>[2x]MGSSHHHHHSSGLVPRGSHMQMIAEIYYERGTIVVKGDAHVPHAKFDSRSGTYRALAFRYRDIIEYFESNGIEFVDNAADPIPTPYFDAEISLRDYQEKALERWLVDKRGCIVLPTGSGKTHVAMAAINELSTPTLIVVPTLALAEQWKERLGIFGEEYVGEFSGRIKELKPLTVSTYDSAYVNAEKLGNRFMLLIFDEVHHLPAESYVQIAQMSIAPFRLGLTATFEREDGRHEILKEVVGGKVFELFPDSLAGKHLAKYTIKRIFVPLAEDERVEYEKREKVYKQFLRARGITLRRAEDFNKIVMASGYDERAYEALRAWEEARRIAFNSKNKIRKLREILERHRKDKIIIFTRHNELVYRISKVFLIPAITHRTSREEREEILEGFRTGRFRAIVSSQVLDEGIDVPDANVGVIMSGSGSAREYIQRLGRILRPSKGKKEAVLYELISRGTGEVNTARRRKNAAKGAA;>MLPKELLDVRRAKGRIFPKFADERDYELAEKVIEIFKKGLGKKYGNLMKQARKLENAKNFKKVRGFIRVLENHCIEKSCAFDVDSELEPRKVRMLLFEHGFVTSKKERDRVLEYVARYFSTTPETVERAMYADREEELILTKFRPLTPDNLIKLYNLSLLQTTLFNALRLTFWASDRHKEIFRSIKRLGLMYELYEDSGRLMVEVTGAATLLKMTRKYGVSFAKLIPWILRAKNWFIRAEISDFDRLYIMEIDDRIRDLFPDVEERLSYDSTLEEEFARKMQMLGYEVEREPDVVKAGKYAFIPDFAVNLGDKKVYIEIAGFWTDEYLRKKAEKIKSSSIPLILIAREDFGDGGANVKDVILFSRKIPYGEVIKALKRYKPEKKVEGDVVELENFAEVPSEYVIAGKYAVRREIFEEIKREIEVSNPSTLEDIKAILKKYGLGESAIRAFGYRVRWIGLGEAVIERTD[2x]

Xeroderma pigmentosum type B (XPB) gene encodes a superfamily 2 (SF2) DNA helicase conserved from archaea to human (1–8). XPB plays a key role in DNA opening at damage sites and coordinating damage incision by nucleases. An XPG-like nuclease, named Bax1, has been reported to form a heterodimer with XPB in many archaea. Furthermore, XPB and Bax1 nuclease have been reported to work together to unwind and cleave DNA substrates resembling NER intermediate DNA structures.

The crystal structure was determined to 3.0 Å resolution by molecular replacement combined with anomalous data obtained from an isomorphous crystal of AfXPB complexed with a Se-Met derivative AfBax1. There are two copies of the AfXPB–Bax1 heterodimer in the asymmetry unit forming a heart-shape. The two AfBax1 molecules interact with each other through the C-termini, particularly, the β-strand loop β-strand (βLβ) C-terminal tails forming two pairs of anti-paralleled β-strands. The two AfXPB molecules remain the open conformation observed in the AfXPB crystal structure. The AfXPB–Bax1 complex structure reveals that AfBax1 exclusively interacts with the C-terminal half XPB including the ThM and HD2. The crystal structure of the AfXPB–Bax1 complex reveals that AfBax1 consists of four domains: the N-terminal domain (NTD), a central domain (CRD), the nuclease (NUS) domain and the C-terminal domain (CTD). The NTD is mainly responsible for the interactions with XPB: the β-hairpin and the first tri-helix bundle (α1–3) interact with the ThM domain of XPB while the second tri-helix bundle (α4–6) interacts with the HD2 of XPB. In contrast, AfBax1 reduces the ATPase activity of AfXPB by 50% instead because the AfXPB–Bax1 heterodimer keeps AfXPB in the open conformation and hinder AfXPB from forming the closed conformation required for ATP binding as the C-terminal half of AfXPB collides with the CRD and NUS domains of AfBax1 when the closed conformation of AfXPB is docked onto the complex structure. Interestingly, the inhibitory effect of AfBax1 on the XPB ATPase activity is removed by Y-shaped or bubbled DNA substrates, which allow the AfXPB–Bax1 complex to have higher ATPase activity than AfXPB alone, suggesting these NER intermediate DNA substrates activate the AfXPB–Bax1 complex, in agreement with its role in nucleotide excision repair.1-METHYLAMINE-1-BENZYL-CYCLOPENTANE | C12 H17 N | 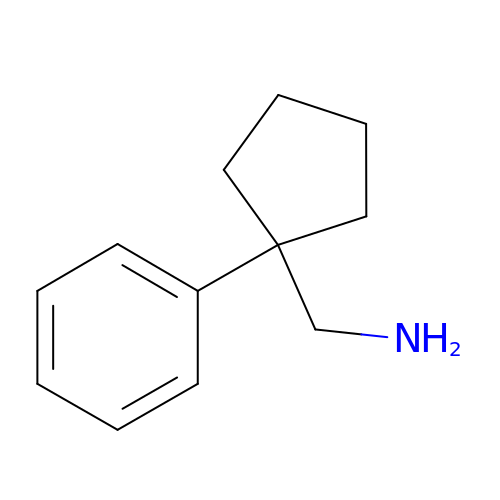SJWOFBVBNFLWLP-UHFFFAOYSA-N> GLP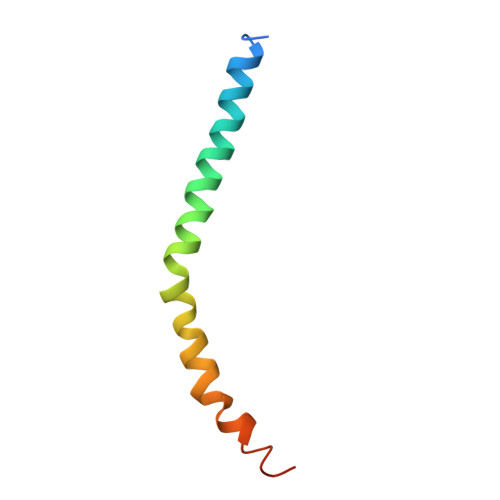RHSAVMERLRRRIELCRRHHSTCEARYEAVSPERLELERQHTFALHQRCIQAKAKRAGKH> MEVEQTSVRSDTNSTCEYLDAEGDPESPNLYQEADPDQEAEQQNHSIISELRDGLGTMRDNSALSPEPGQENKGLAASVESLALSTSTSAKTEDSIGGGLEEEYDYQHDSLWQGQKKHIFILSEAGKPIFSLHGNEDKLATLFGVIQALVSFVQMGQDAITSIHAGGIKFAFMQRSSLILVAASRSNMSVQQLQLQLGDVYNQILSILTYSHMTKIFERRKNFDLRRLLSGSERLFYNLLANDSSSAKVSNNIFTFLTNSIRVFPLPTTIRSQITSAIQSNCSKIKNLVFAVLIANNKLIALVRMKKYSIHPADLRLIFNLVECSESFKSSENWSPICLPKFDMN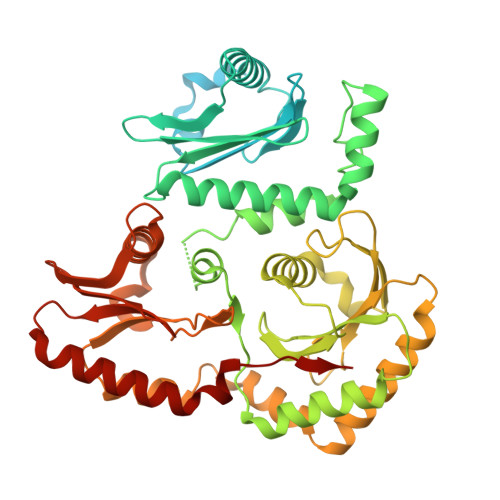GYLHAHVSYLADDCQACLLLLSVDRDAFFTLAEAKAKITEKLRKSHCLEAINEELQQPFNAKLYQQVVGIPELRHFLYKPKSTAQLLCPMLRHPYKSLTELERLEAIYCDLLHRIHNSSRPLKLIYEMKEREVVLAWATGTYELYAIFEPVVDKATVIKYVDKLIKWIEKEYDVYFIRNHATF> MKLTLWTYEGPPHVGAMRVATAMKDLQLVLHGPQGDTYADLLFTMIERRNARPPVSFSTFEASHMGTDTAILLKDALAAAHARYKPQAMAVALTCTAELLQDDPNGISRALNLPVPVVPLELPSYSRKENYGADETFRALVRALAVPMERTPEVTCNLLGATALGFRHRDDVAEVTKLLATMGIKVNVCAPLGASPDDLRKLGQAHFNVLMYPETGESAARHLERACKQPFTKIVPIGVGATRDFLAEVSKITGL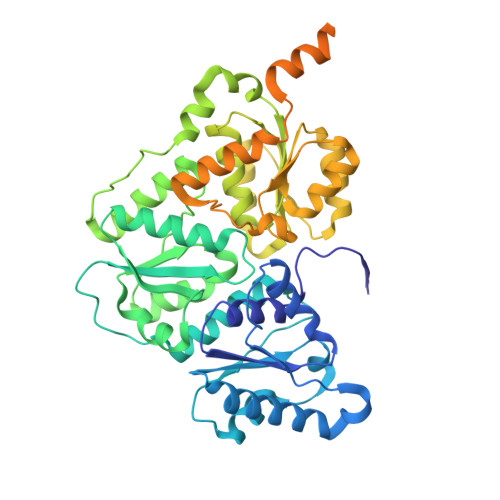PVVTDESTLRQPWWSASVDSTYLTGKRVFIFGDGTHVIAAARIAAKEVGFEVVGMGCYNREMARPLRTAAAEYGLEALITDDYLEVEKAIEAAAPELILGTQMERNIAKKLGLPCAVISAPVHVQDFPARYAPQMGFEGANVLFDTWVHPLVMGLEEHLLTMFREDFEFHDAAGASHHGGKAVAREESPVAPADLAPAATSDTPAAPSPVVVTQASGEIRWMPEAERELRKIPFFVRGKAKRNTELYAAHKGVCDITVETLYEAKAHYAR In epithelial tissues, the cadherin intracellular domain binds to β-catenin, which in turn associates with the F-actin-binding protein αE-catenin. Specifically, αE-catenin functions as a force-sensitive structural switch that displays two-state catch bond behavior: it transitions from weak to strong actin-binding states between low (<2 pN) and moderate (8 pN) forces. The structure of αE-catenin comprises a series of α-helical bundles organized into three main regions: an N-terminal (N) domain that consists of two four-helix bundles (NI and NII) that both binds β-catenin and mediates homodimerization; a middle (M) domain consisting of three four-helix bundles (MI, MII, and MIII) that harbor binding sites for vinculin and other protein partners; and a C-terminal, five-helix bundle termed the actin-binding domain (ABD)18,26. The interactions of αE-catenin are allosterically modulated by binding to its protein partners and by mechanical load.

Therefore, we determined the crystal structure of the αE-catenin 82–883 dimer at 4.0 Å resolution without dehydration, and also examined its structure in solution by SAXS. The ABDs in αE-catenin 82–883 crystals were disordered, and the protein is extended in solution, demonstrating that the disorder of the ABDs and the extended nature of the molecule are not due to the absence of the first 81 residues. Superposition of the individual protomers in each αE-catenin dimer crystal structure shows that although the N- and M- domains have similar structures, they assume two different orientations with respect to each other due to differences in the N-M interface formed by the NII and MII bundles. Cysteine labeling provided evidence for this coupling: upon binding to E-cadherin•β-catenin to NI, C228 in NII becomes significantly more exposed in αE-catenin. C228 packs against Y237, which is directly in the interface with MII, so changes in its exposure may arise from changes in the NII-MII interface. Murine αE-catenin has 12 cysteine residues, which the crystal structures reveal have variable levels of solvent exposure. Mass spectrometry revealed variable levels of mBBr incorporation at the different sites that correlated only weakly with Cys side chain exposure observed in crystal structures. This may reflect dynamics of the molecule in solution vs. the conformation observed in crystal structures. Notably, Cys 324 and Cys 337 in MI, which have limited solvent accessibility in crystal structures, label strongly; this region is also proteolytically sensitive, indicating that MI is relatively unstable and flexible.

>GGILESQFLKEELVVAVEDVRKQGDLMKSAAGEFADDPSSSVKRGNMVRAARALLSAVTRLLILADMADVYKLLVQLKVVEDGILKLRNAGNEQDLGIQYKALKPEVDKLNIMAAKRQQELKDVGNRDQMAAARGILQKNVPILYTASQACLQHPDVAAYKANRDLIYKQLQQAVTGISNAAQATASDDAAQHQGGSGGELAYALNNFDKQIIVDPLSFSEERFRPSLEERLESIISGAALMADSSCTRDDRRERIVAECNAVRQALQDLLSEYMGNAGRKERSDALNSAIDKMTKKTRDLRRQLRKAVMDHVSDSFLETNVPLLVLIEAAKNGNEKEVKEYAQVFREHANKLIEVANLACSISNNEEGVKLVRMSASQLEALCPQVINAALALAAKPQSKLAQENMDLFKEQWEKQVRVLTDAVDDITSIDDFLAVSENHILEDVNKCVIALQEKDVDGLDRTAGAIRGRAARVIHVVTSEMDNYEPGVYTEKVLEATKLLSNTVMPRFTEQVEAAVEALSSDPAQPMDENEFIDASRLVYDGIRDIRKAVLMIRTPEELDDSDFETEDFDVRSRTSVQTEDDQLIAGQSARAIMAQLPQEQKAKIAEQVASFQEEKSKLDAEVSKWDDSGNDIIVLAKQMCMIMMEMTDFTRGKGPLKNTSDVISAAKKIAEAGSRMDKLGRTIADHCPDSACKQDLLAYLQRIALYCHQLNICSKVKAEVQNLGGELVVSGVDSAMSLIQAAKNLMNAVVQTVKASYVASTKYQKSQGMASLNLPAVSWKMKAPEKKPLVKREKQDETQTKIK[2x]>[2x]GSMDQRQKLQHWIHSCLRKADKNKDNKMNFKELKDFLKELNIQVDDGYARKIFRECDHSQTDSLEDEEIETFYKMLTQRAEIDRAFEEAAGSAETLSVERLVTFLQHQQREEEAGPALALSLIERYEPSETAKAQRQMTKDGFLMYLLSADGNAFSLAHRRVYQDMDQPLSHYLVSSSHNTYLLEDQLTGPSSTEAYIRALCKGCRCLELDCWDGPNQEPIIYHGYTFTSKILFCDVLRAIRDYAFKASPYPVILSLENHCSLEQQRVMARHLRAILGPILLDQPLDGVTTSLPSPEQLKGKILLKGKKLGGLLPAGGENGSEATDVSDEVEAAEMEDEAVRSQVQHKPKEDKLKLVPELSDMIIYCKSVHFGGFSSPGTSGQAFYEMASFSESRALRLLQESGNGFVRHNVSCLSRIYPAGWRTDSSNYSPV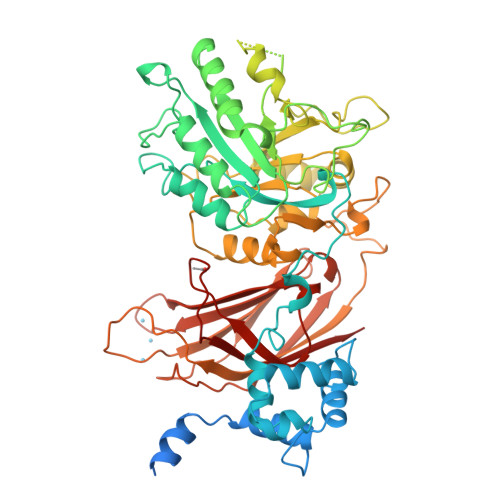EMWNGGCQIVALNFQTPGPEMDVYLGCFQDNGGCGYVLKPAFLRDPNTTFNSRALTQGPWWRPERLRVRIISGQQLPKVNKNKNSIVDPKVIVEIHGVGRDTGSRQTAVITNNGFNPRWDMEFEFEVTVPDLALVRFMVEDYDSSSKNDFIGQSTIPWNSLKQGYRHVHLLSKNGDQHPSATLFVKISIQD>[2x]MTFTVFTGGDSGAWSILSVAPVIGESLMAASHLAIAPSLSLGDTSATTPWQLRGVASHARYVERAEKIALTSVQAGLGRNEATRAALIPIRKSAAWWEMTQDERRAIFEDKSHHIAAS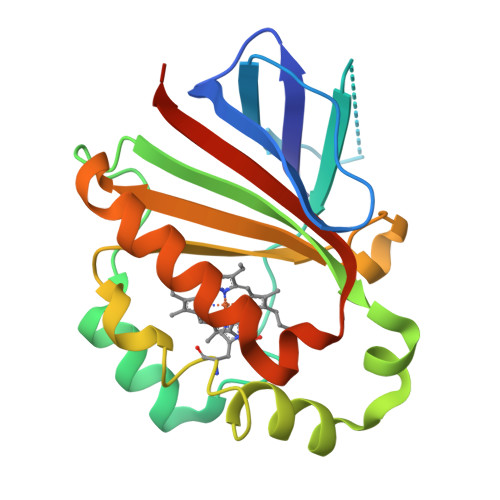LKYLPAIARQLYHCRDIGEPFDFLTWFEYAPEHATMFEDLVGVLRATEEWTYVEREVDIRLARAIHHHHHH>DVYTDHGDLYNTPVRMLVVAGAKFKEALKPWLTWKAQKGFYLDVHYTDEAEVGTTNASIKAFIHKKYNDGLAASAAPVFLALVGDTDVISGEKGKKTKKVTDLYYSAVDGDYFPEMYTFRMSASSPEELTNIIDKVLMYEKATMPDKSYLEKVLLIAGADYSWNSQVGQPTIKYGMQYYYNQEHGYTDVYNYLKAPYTGCYSHLNTGVSFANYTAHGSETAWADPLLTTSQLKALTNKDKYFLAIGNCCITAQFDYVQPCFGEVITRVKEKGAYAYIGSSPNSYWGEDYYWSVGANAVFGVQPTFEGTSMGSYDATFLEDSYNTVNSIMWAGNLAATHAGN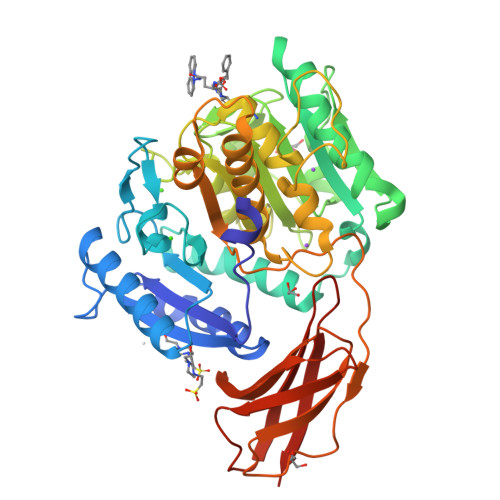IGNITHIGAHYYWEAYHVLGDGSVMPYRAMPKTNTYTLPASLPQNQASYSIQASAGSYVAISKDGVLYGTGVANASGVATVSMTKQITENGNYDVVITRSNYLPVIKQIQVGEPHHHHHH[2x]>[8x]MDPFASTRTFNLAMTDIGEMYFMPPLMEALAQRAPHIQISTLRPNAGNLKEDMESGAVDLALGLLPELQTGFFQRRLFRHRYVCMFRKDHPSAKSPMSLKQFSELEHVGVVALNTGHG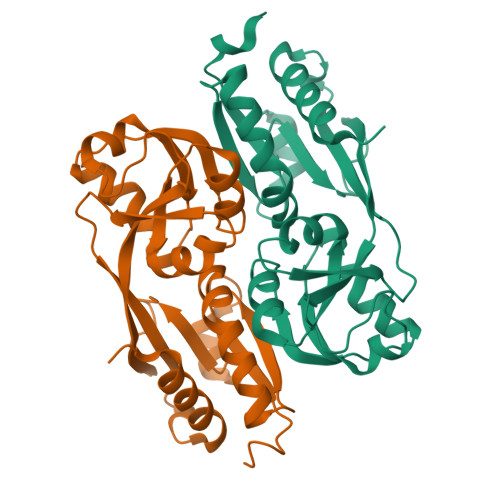EVDGLLERAGIKRRMRLVVPHFIAIGPILHSTDLIATVPQRFAVRCEVPFGLTTSPHPAKLPDIAINLFWHAKYNRDPGNMWLRQLFVELFSEAHHHHHH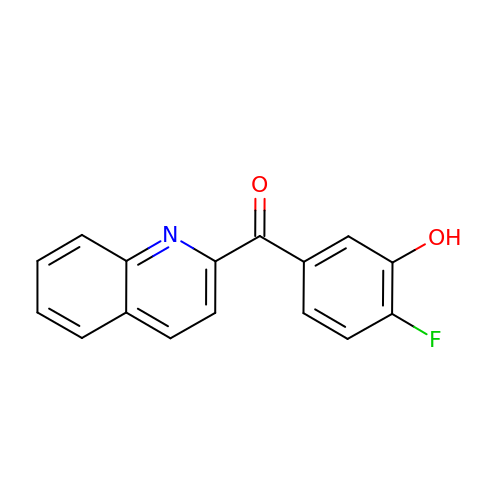(4-fluoranyl-3-oxidanyl-phenyl)-quinolin-2-yl-methanone | C16 H10 F N O2 | JNWWABLECBACFV-UHFFFAOYSA-N> MADYKDDDDKSGPDEVDASGRMGFVRQIQLLLWKNWTLRKRQKIRFVVELVWPLSLFLVLIWLRNANPLYSHHECHFPNKAMPSAGMLPWLQGIFCNVNNPCFQSPTPGESPGIVSNYNNSILARVYRDFQELLMNAPESQHLGRIWTELHILSQFMDTLRTHPERIAGRGIRIRDILKDEETLTLFLIKNIGLSDSVVYLLINSQVRPEQFAHGVPDLALKDIACSEALLERFIIFSQRRGAKTVRYALCSLSQGTLQWIEDTLYANVDFFKLFRVLPTLLDSRSQGINLRSWGGILSDMSPRIQEFIHRPSMQDLLWVTRPLMQNGGPETFTKLMGILSDLLCGYPEGGGSRVLSFNWYEDNNYKAFLGIDSTRKDPIYSYDRRTTSFCNALIQSLESNPLTKIAWRAAKPLLMGKILYTPDSPAARRILKNANSTFEELEHVRKLVKAWEEVGPQIWYFFDNSTQMNMIRDTLGNPTVKDFLNRQLGEEGITAEAILNFLYKGPRESQADDMANFD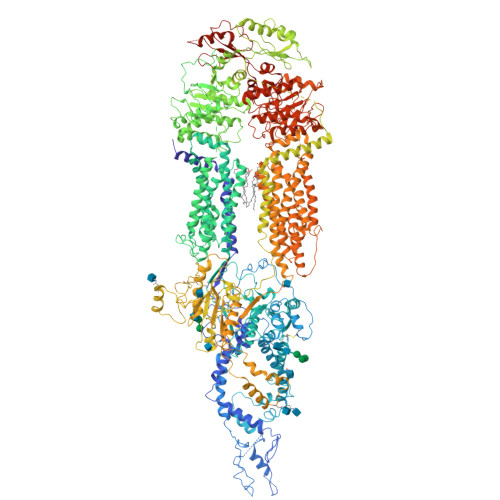WRDIFNITDRTLRLVNQYLECLVLDKFESYNDETQLTQRALSLLEENMFWAGVVFPDMYPWTSSLPPHVKYKIRMDIDVVEKTNKIKDRYWDSGPRADPVEDFRYIWGGFAYLQDMVEQGITRSQVQAEAPVGIYLQQMPYPCFVDDSFMIILNRCFPIFMVLAWIYSVSMTVKSIVLEKELRLKETLKNQGVSNAVIWCTWFLDSFSIMSMSIFLLTIFIMHGRILHYSDPFILFLFLLAFSTATIMLCFLLSTFFSKASLAAACSGVIYFTLYLPHILCFAWQDRMTAELKKAVSLLSPVAFGFGTEYLVRFEEQGLGLQWSNIGNSPTEGDEFSFLLSMQMMLLDAAVYGLLAWYLDQVFPGDYGTPLPWYFLLQESYWLGGEGCSTREERALEKTEPLTEETEDPEHPEGIHDSFFEREHPGWVPGVCVKNLVKIFEPCGRPAVDRLNITFYENQITAFLGHNGAGKTTTLSILTGLLPPTSGTVLVGGRDIETSLDAVRQSLGMCPQHNILFHHLTVAEHMLFYAQLKGKSQEEAQLEMEAMLEDTGLHHKRNEEAQDLSGGMQRKLSVAIAFVGDAKVVILDEPTSGVDPYSRRSIWDLLLKYRSGRTIIMSTHHMDEADLLGDRIAIIAQGRLYCSGTPLFLKNCFGTGLYLTLVRKMKNIQSQRKGSEGTCSCSSKGFSTTCPAHVDDLTPEQVLDGDVNELMDVVLHHVPEAKLVECIGQELIFLLPNKNFKHRAYASLFRELEETLADLGLSSFGISDTPLEEIFLKVTEDSDSGPLFAGGAQQKRENVNPRHPCLGPREKAGQTPQDSNVCSPGAPAAHPEGQPPPEPECPGPQLNTGTQLVLQHVQALLVKRFQHTIRSHKDFLAQIVLPATFVFLALMLSIVIPPFGEYPALTLHPWIYGQQYTFFSMDEPGSEQFTVLADVLLNKPGFGNRCLKEGWLPEYPCGNSTPWKTPSVSPNITQLFQKQKWTQVNPSPSCRCSTREKLTMLPECPEGAGGLPPPQRTQRSTEILQDLTDRNISDFLVKTYPALIRSSLKSKFWVNEQRYGGISIGGKLPVVPITGEALVGFLSDLGRIMNVSGGPITREASKEIPDFLKHLETEDNIKVWFNNKGWHALVSFLNVAHNAILRASLPKDRSPEEYGITVISQPLNLTKEQLSEITVLTTSVDAVVAICVIFSMSFVPASFVLYLIQERVNKSKHLQFISGVSPTTYWVTNFLWDIMNYSVSAGLVVGIFIGFQKKAYTSPENLPALVALLLLYGWAVIPMMYPASFLFDVPSTAYVALSCANLFIGINSSAITFILELFENNRTLLRFNAVLRKLLIVFPHFCLGRGLIDLALSQAVTDVYARFGEEHSANPFHWDLIGKNLFAMVVEGVVYFLLTLLVQRHFFLSQWIAEPTKEPIVDEDDDVAEERQRIITGGNKTDILRLHELTKIYPGTSSPAVDRLCVGVRPGECFGLLGVNGAGKTTTFKMLTGDTTVTSGDATVAGKSILTNISEVHQNMGYCPQFDAIDELLTGREHLYLYARLRGVPAEEIEKVANWSIKSLGLTVYADCLAGTYSGGNKRKLSTAIALIGCPPLVLLDEPTTGMDPQARRMLWNVIVSIIREGRAVVLTSHSMEECEALCTRLAIMVKGAFRCMGTIQHLKSKFGDGYIVTMKIKSPKDDLLPDLNPVEQFFQGNFPGSVQRERHYNMLQFQVSSSSLARIFQLLLSHKDSLLIEEYSVTQTTLDQVFVNFAKQQTESHDLPLHPRAAGASRQAQDLEGSDEVDAVEGSHHHHHHHHHH> MSTLADQALHNNNVGPIIRAGDLVEPVIETAEIDNPGKEITVEDRRAYVRIAAEGELILTRKTLEEQLGRPFNMQELEINLASF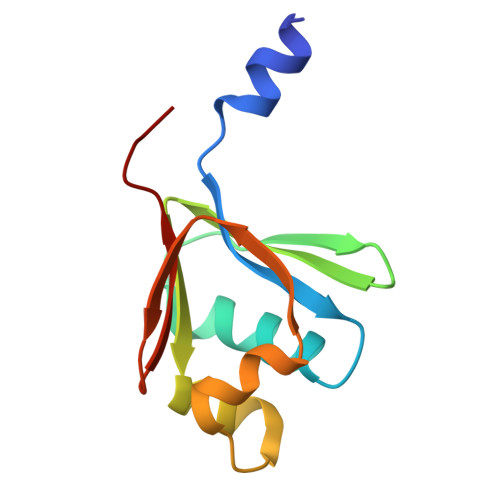AGQIQADEDQIRFYFDKTM> GELRVGLEESELWLRFKELTNEMIVTKNGRRMFPVLKVNVSGLDPNAMYSFLLDFVAADNHRWKYVNGEWVPGGKPEPQAPSCVYIHPDSPNFGAHWMKAPVSFSKVKLTNKLNGGGQIMLNSLHKYEPRIHIVRVGDPQRMITSHCFPETQFIAVTAYQNEEITALKIKYN

Brachyury is a transcription factor that plays an essential role in tumour growth of the rare bone cancer chordoma and is implicated in other solid tumours. Brachyury (encoded by the TBXT gene, also formerly known as T) is the founding member of the family and was first identified in 19275. The DNA binding domain forms an immunoglobulin-like fold and contacts DNA via an unusual insertion of an α-helix into the minor groove. All T-box proteins recognize a common consensus sequence named the T-box binding element (AGGTGTGAAA) with family member-specific variations found in the preferences for repeats, orientations (inverted or tandem), and spacing of such repeats.

For X-ray fragment screening in the absence of DNA, we used a shorter construct (amino acids 41–211) lacking the C-terminal helix that inserts into the DNA minor groove, which was observed to be flexible in our early DNA-free crystallization efforts. WT and G177D DNA-free crystals were obtained in different conditions with different crystal forms although both generally diffracted to around 1.6 Å. The structures of WT and G177D brachyury in the absence of DNA are almost identical to their counterparts bound to DNA (R.M.S.D. 0.36 and 0.37, respectively), including the significant differences observed around the G177D variant despite different crystal packing interactions, thus validating that these differences are not crystallographic artifacts. Encouraged by the discovery of ligandable pockets on brachyury, we have initiated a medicinal chemistry campaign to optimize the potency of fragment-derived molecules.>GSKKHTGYVGLKNQGATCYMNSLLQTLFFTNQLRKAVYMMPTEGDDSSKSVPLALQRVFYELQHSDKPVGTKKLTKSFGWETLDSFMQHDVQELCRVLLDNVENKMKGTCVEGTIPKLFRGKMVSYIQCKEVDYRSDRREDYYDIQLSIKGKKNIFESFVDYVAVEQLDGDNKYDAGEHGLQEAEKGVKFLTLPPVLHLQLMRFMYDPQTDQNIK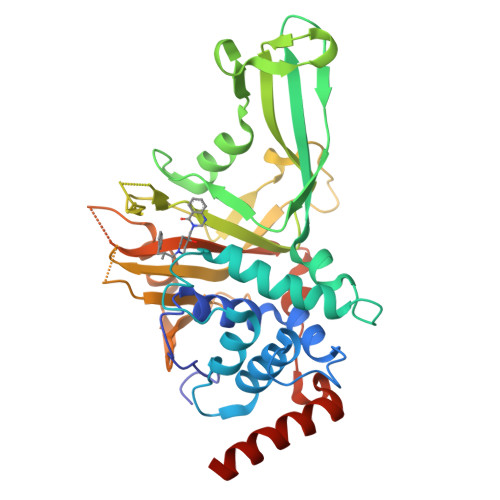INDRFEFPEQLPLDEFLQKTDPKDPANYILHAVLVHSGDNHGGHYVVYLNPKGDGKWCKFDDDVVSRCTKEEAIEHNYGGHDDDLSVRHCTNAYMLVYIRESKLSEVLQAVTDHDIPQQLVERLQEEKRIEAQKRKERQE[2x]> MKVRVDADACIGCGVCENLCPD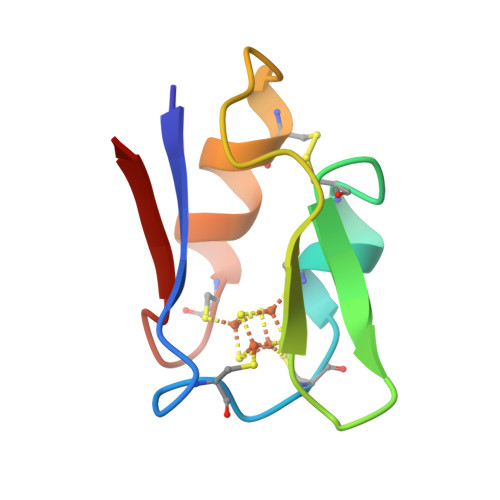VFQLGDDGKAKVLQPETDLPCAKDAADSCPTGAISVEE>[2x]MQERRALRLGVNGLPNSLEPVNAISNVGPRIVNQIFDTLIARDFFAKGAPGNAIDLVPALAESWERIDEKSVRFKLRQKVMFHDGVELTADDVAYTFSSERLWGPEAIKKIPLGKSYSLDFDEPVVEDKYTVTLRTKTPSYLIETFVASWMSRIVPKEYYKKLGAVDFGNKP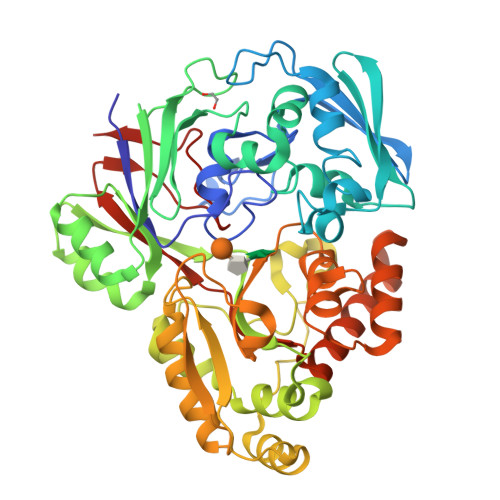VGTGPYKFVEFVAGDRVVLEANDAYWGPKPTASKITYQIVAEPATRVAGLISGEYDIITTLTPDDIQLINSYPDLETRGTLIENFHMFTFNMNQEVFKDKKLRRALALAVNRPIMVEALWKKQASIPAGFNFPNYGETFDPKRKAMEYNVEEAKRLVKESGYDGTPITYHTMGNYYANAMPALMMMIEMWKQIGVNVVMKTYAPGSFPPDNQTWMRNWSNGQWMTDAYATIVPEFGPNGQVQKRWGWKAPAEFNELCQKVTVLPNGKERFDAYNRMRDIFEEEAPAVILYQPYDVYAARKDVHWKPVSFEMMEFRNNLSFGHHHHHH> MSLSSWRQFQLFENIPIRDPNFGGDSLLYSDPTLCAATIVDPQTLIIAVNSNIIKVVKLNQSQVIHEFQSFPHDFQITFLKVINGEFLVALAESIGKPSLIRVYKLEKLPNREQLYHSQVELKNGNNTYPISVVSISNDLSCIVVGFINGKIILIRGDISRDRGSQQRIIYEDPSKEPITALFLNNDATACFAATTSRILLFNTTGRNRGRPSLVLNSKNGLDLNCGSFNPATNEFICCLSNFIEFFSSSGKKHQFAFDLSLRKRIFCVDKDHILIVTEETGVPTTSISVNELSPTIINRIFIIDAKNKIISLNFVVSSAIIDIFSTSQSGKNITYLLTSEGVMHRITPKSLENQINIIIQKELYPFALQLAKQHSLSPLDVQEIHKKYGDYLFKKGLRKEATDQYIQCLDVVETSEIISKFGVKEVPDPESMRNLADYLWSLIKNSISQRDHVTLLLIVLIKLKDVEGIDTFIQHFDRKGIWNEGVVMDDMDDVTFFYS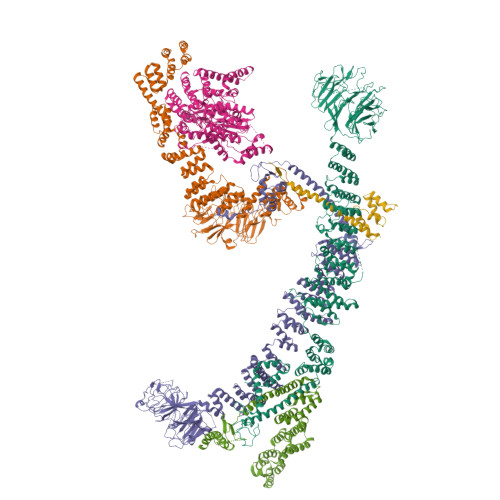DNDFFDLDLILELMKESDFKRLSYRLAKKYSKDSLIIVDILLNLLHNPVKAIKYIKSLPIDETLRCLVTYSKKLLEESPNETNALLIEVFTGKFKPSTFEVDLDRRDTTGDFSENIRTVFYSYKTFFNYMNSNGTSDAMSESSEASHEHEEPTYHPPKPSIVFSSFVTKPFEFVVFLEACLACYQQYEGFDEDRQVILTTLYDLYLNLAQNDVPERIDDWRSRATGVLRESNKLVYSAASNNTSKRVDNSIMLLISHMDQSSASAKDKTKIDIASFANDNPEMDLLSTFRAMTLNEEPSTCLKFLEKYGTEEPKLLQVALSYFVSNKLIFKEMGGNEVLKEKVLRPIIEGERMPLLDIIKALSRTNVAHFGLIQDIIIDHVKTEDTEIKRNEKLIESYDKELKEKNKKLKNTINSDQPLHVPLKNQTCFMCRLTLDIPVVFFKCGHIYHQHCLNEEEDTLESERKLFKCPKCLVDLETSNKLFEAQHEVVEKNDLLNFALNSEEGSRDRFKVITEFLGRGAISYSDITI;> MKNPSFDWERLKDVFYRSRAIGELKWPTQYEEFKCALSLTVIAVEIQDFIQVYNYFGQLLGKINLQRIHEDIIKFEFDKDEKLILVTKSSIKIVKGWSPLTIESVPLQDPTIDTIWDYHNGIMLLAKSRDIYKLNGNEWELLYENKDKKYNLLTKNHWSCNDDSIILLDVDHVYQVSTSNGALLKLITDSSWHKVTISSRGFICLYNMKDNKLQIFRDPARILMEHNLDSTPDDICWCGNDTVACSFEDEIKLYGPDGLYVTFWYPFTVTNLRAEVDGLKVITTEKIYFLSRVQPQTSNIFRIGSTEPGAMLVDSFSLLEDHAPKAIEILKNFVLEKGVLDCIAAAIDEFEPKLQKMLLNAASYGKASLQYKSFDASIFVNACNTIKLLNCFRSFGIFLTVEEYRCISLKGVIDRLLKYHRYYECIQICKLANERFLLGYVFTEWAKDKIKGSPDMEDDELLDKIKSRLSVIDMTDTLQMVAVAKVAYLEGRFQLSRNLALLEKNEEARIEQLYNLDDDSIALKECIKVQNYSLTISLLIALSKKLTNSQLTKLLIIDMFNNPLYLYYMRMDKAYLYDFYRQTDRFIDLAHVLLQQGKEQQSLHSFLPQIKDLYSQVQNSEVVNNTIEQLQRQEKLWIYQESLGKRFAISFTNMTLDQTLSKLIETGQDKQVKEIVKKFKISEKKLYHLKCKTLVEAKKFDELLQFAQSRKSPIGYMPFYTYLKSRGHMDKASPYVNMIPGLSYQEKKKLYVECRGFRDAIQLAGKEKDIPGLKEIYNIIPPNEPELKALANETMSRI;> MIKTRIEEVQLQFLTGNTELTHLKVSNDQLIVTTQRTIYRINLQDPAIVNHFDCPLSKELETIMNVHVSPMGSVILIRTNFGRYMLLKDGEFTQLNKIKNLDLSSLHWINETTFLMGIKKTPKLYRVELTGKDITTKLWYENKKLSGGIDGIAYWEGSLLLTIKDNILYWRDVTNMKFPLVLPDESEQFERLKHHAIKKFDSYNGLFAWVTSNGIVFGDLKEKQMEKDPASNNFGKFLSSSKVLLNFELPDYQNDKDHLIKDIVLTAFHILLLRKNTVTMVSQLNNDVVFHETIPRHQLTGSNTDSNEKFLGLVRDSVKETFWCFSNINVFEIIIENEPNSVWNLLVRDNKFDKALSLKGLTVREIESVKLSKAMYLFHTAKDFHSAAQTLGSMKDLSHFGEIALNFLQIKDYNDLNVILIKQLDNVPWKSTQVVLSSWIIWNFMKQLNDIELKINTTKPASTDEDNLLNWNLNLKEKSNELTKFLESHLEKLDNETVYQIMSKQNRQNELLIFASLINDMKFLLSFWIDQGNWYESLKILLTINNHDLVYKYSLILLLNSPEATVSTWMKIKDLDPNKLIPTILKFFTNWQNNSKLITNISEYPENYSLTYLKWCVREVPKMCNPIVYNSILYMMITDPRNDMILENDIIKFMKSNENKYDLNFQLRLSLKFKKTKTSIFLLTRLNLFEDAIDLALKNNLIDDCKVIVNDEILIEDYKLRKRLWLKIAKHLLLSMKDIDIKQLIRTILNDSNEILTIKDLLPFFNEYTTIANLKEELIKFLENHNMKMNEISEDIINSKNLKVEINTEISKFNEIYRILEPGKSCDECGKFLQIKKFIVFPCGHCFHWNCIIRVILNSNDYNLRQKTENFLKAKSKHNLNDLENIIVEKCGLCSDININKIDQPISIDETELAKWNE;> MNRFWNTKKFSLTNADGLCATLNEISQNDEVLVVQPSVLPVLNSLLTFQDLTQSTPVRKITLLDDQLSDDLPSALGSVPQMDLIFLIDVRTSLRLPPQLLDAAQKHNLSSLHIIYCRWKPSFQNTLEDTEQWQKDGFDLNSKKTHFPNVIESQLKELSNEYTLYPWDLLPFPQIDENVLLTHSLYNMENVNMYYPNLRSLQSATESILVDDMVNSLQSLIFETNSIITNVVSIGNLSKRCSHLLKKRIDEHQTENDLFIKGTLYGERTNCGLEMDLIILERNTDPITPLLTQLTYAGILDDLYEFNSGIKIKEKDMNFNYKEDKIWNDLKFLNFGSIGPQLNKLAKELQTQYDTRHKAESVHEIKEFVDSLGSLQQRQAFLKNHTTLSSDVLKVVETEEYGSFNKILELELEILMGNTLNNDIEDIILELQYQYEVDQKKILRLICLLSLCKNSLREKDYEYLRTFMIDSWGIEKCFQLESLAELGFFTSKTGKTDLHITTSKSTRLQKEYRYISQWFNTVPIEDEHAADKITNENDDFSEATFAYSGVVPLTMRLVQMLYDRSILFHNYSSQQPFILSREPRVSQTEDLIEQLYGDSHAIEESIWVPGTITKKINASIKSNNRRSIDGSNGTFHAAEDIALVVFLGGVTMGEIAIMKHLQKILGKKGINKRFIIIADGLINGTRIMNSIS;> MLRAQKLHSLKSSDITAILPTEQSQKLVLAKKNGDVEVYSRDGNTLKLFQVYPDLLQNAKNDPLPPVIENFYFANELSTIFAQCKETLILLSTTNLHEYDRIIDRRGINHCWLFERSHKNKEEKNTYLIYSTINTAKMRVLIWEGRTYKNMMEASLSYRKETIRSIYPGETGITLATDLGIYHWPYNKPSLIRIEKTVKNKFPKDMISALTELKEQAEKVIEKKPKKNSHFDAQSFSSMDRMSRKSSMSSLWYRTIRNERGNKIRYTFELDGNDATPMIIDGATKKIFKVELMHNNEEPFLIATDHATFSESNSEFDHMQYLSSNLLMLYNSSTIKFVDYENGFTFLQQKIPEGIKWVKNLSGTYFLVWTSNDEVQLFSYHVDDGSEDDDQESICGDINDPDFYQLWRKVLFYKFFIDSPHSKELCVSDNPEESLDICAMKLRDLTVMWCLRIFDKFQNYMVQLERSRNSRMIRSKCEEMIIKSIFDLFIKFWAPPQLVILKVFPSAISSLVLEITGQEHHCLLKEAEEVKETYDIPPHLLNRWCLPYLTDTRRHLQNLLSKENDDESRITWCYRDREIKQSFDFFLISNHDDVDLNTMLTLIDTVLFKCYLYYNPPMVGPFIRVENHCDSHVIVTELKIRHMFKDLIDFYYKRGNHEEALKFLTDLVDELENDNTDQKQRQKIDHGVKILVIYYLKKLSNPQLDVIFTYTDWLLNRHNDSIKEILSSIFFYDSQACSSRDHLKVYGYIKKFDKLLAIQYLEFAISTFRLEGNKLHTVLIKLYLENLDIPSTRIKLKSLLETTSVYEPRTILKLLNDAIESGSDQLPTNQLNFVKYLKIFPLSKLENHKEAVHILLDEIDDYKAATSYCNDVYQSDSTKGEELLLYLYSKLVSIYDSNRNSKLILNFLQDHGSKLNSAEIYKNLPQDISLYDIGRVVSQLLKKHTSKMDETRLEKALLQVELVATTYKLNERMSSYGVLSDSHKCPICKKVISNFGTDSISWFTREGRNIITHYNCGKVLQERFNAKNEKSSRIKQKTLGEVINELNNK;> MTTDNHQNDSVLDQQSGERTIDESNSISDENNVDNKREDVNVTSPTKSVSCISQAENGVASRTDESTITGSATDAETGDDDDDDDDDDDEDEDDEDEPPLLKYTRISQLPKNFFQRDSISSCLFGDTFFAFGTHSGILHLTTCAFEPIKTIKCHRSSILCINTDGKYFATGSIDGTVIIGSMDDPQNITQYDFKRPINSVALHSNFQASRMFVSGGMAGDVVLSQRNWLGNRIDIVLNKKKKKKTRKDDLSSDMKGPIMGIYTMGDLILWMDDDGITFCDVPTRSQLLNIPFPSRIFNVQDVRPDLFRPHVHFLESDRVVIGWGSNIWLFKVSFTKDSNSIKSGDSNSQSNNMSHFNPTTNIGSLLSSAASSFRGTPDKKVELECHFTVSMLITGLASFKDDQLLCLGFDIDIEEEATIDEDMKEGKNFSKRPENLLAKGNAPELKIVDLFNGDEIYNDEVIMKNYEKLSINDYHLGKHIDKTTPEYYLISSNDAIRVQELSLKDHFDWFMERKQYYKAWKIGKYVIGSEERFSIGLKFLNSLVTKKDWGTLVDHLNIIFEETLNSLDSNSYDVTQNVLKEWADIIEILITSGNIVEIAPLIPKKPALRKSVYDDVLHYFLANDMINKFHEYITKWDLKLFSVEDFEEELETRIEAASEPTASSKEEGSNITYRTELVHLYLKENKYTKAIPHLLKAKDLRALTIIKIQNLLPQYLDQIVDIILLPYKGEISHISKLSIFEIQTIFNKPIDLLFENRHTISVARIYEIFEHDCPKSFKKILFCYLIKFLDTDDSFMISPYENQLIELYSEYDRQSLLPFLQKHNNYNVESAIEVCSSKLGLYNELIYLWGKIGETKKALSLIIDELKNPQLAIDFVKNWGDSELWEFMINYSLDKPNFTKAILTCSDETSEIYLKVIRGMSDDLQIDNLQDIIKHIVQENSLSLEVRDNILVIINDETKKFANEFLKIRSQGKLFQVDESDIEINDDLNGVLDYKDDDDKDYKDDDDKDYKDDDDK>MRHDFVFSGVIMLELNAKTTALVVIDLQEGILPFAGGPHTADEVVNRAGKLAAKFRASGQPVFLVRVGWSADYAEALKQPVDAPSPAKVLPENWWQHPAALGTTDSDIEIIKRQWGAFYGTDLELQLRRRGIDTIVLCGISTNIGVESTARNAWELGFNLVIAEDACSAASAEQHNNSINHIYPRIARVRSVEEILNA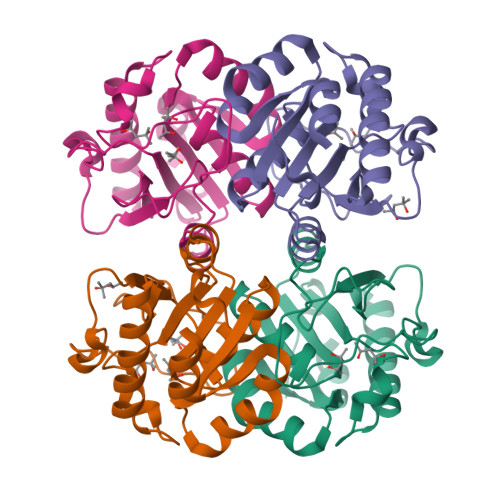L[4x]> GSHMNGFTHYDVVIIGSGPAGSLCGIECRKKGLSVLCIEKEQFPRFHIGESLTGNAGQIIRDLGLAEDMDAAGFPDKPGVNVIGSLSKNEFFIPILAPTWQVRRS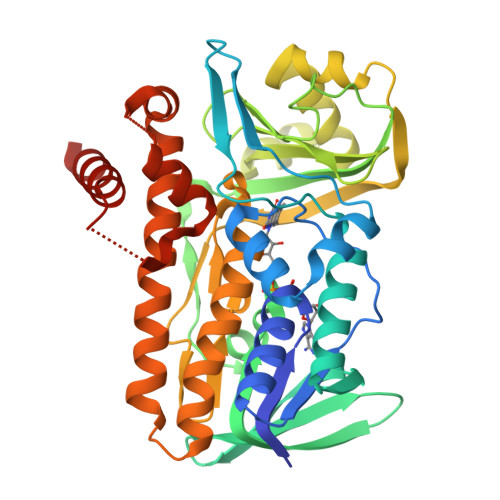DFDDMIKRKAVEHGVEYKLGMVTDVIKDGEKVVGALYKADGVEHQVRSKVLVDASGQNTFLSRKGVAGKRQIEFFSQQIASFAHYKGVERDLPPFSTNTTILYSKQYHWSWIIPISPDTDSLGVVIPKDLYYKECKNPDDAIAWGMDHISPELKRRFKNAERQGDSQSMADFSYRIEPFVGDGWMCIGDAHRFLDPIFSSGVSVAMKEGIRAAEAIAQVVAGQDWKAPFYAYRDWSNGGQQIWADLIRYFWIYPIFFGYQMQNPDLRDEVIRLLGGCCFDCEGWKAPAIFRNAIEEYDRKQMAS>GWVWNQFFVVEEYTGTEPLYVGKIHSDSDEGDGTIKYTISGEGAGTIFLIDELTGDIHATERLDREQKTFYTLRAQARDRATNRLLEPESEFIIKVQDINDSEPRFLHGPYIGSVAELSPTGTSVMQVMASDADDPTYGSSARLVYSVLDGEHHF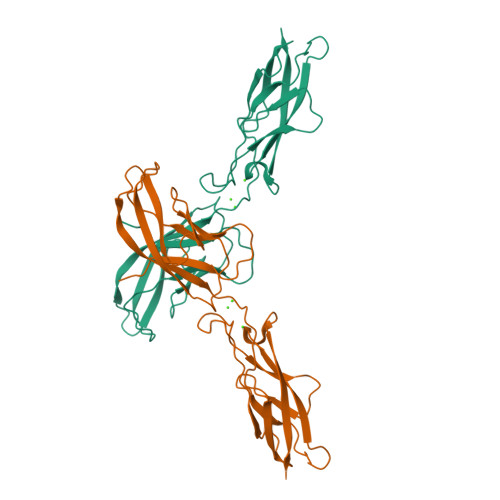TVDPKTGVIRTAVPDLDRESQERYEVVIQATDMAGQLGGLSGSTTVTIVVTD[2x]> MKSRLKQQIFAISLLACTAISPANALQTHLLREQFQNPSDEAKPWTFWYWMFGAVSKEGITADLEAMKRAGLGGTYLMPIKGIKEGPQYNGKAQQLTPEWWEMVRFSMEEADRLGLKLGMHICDGFALAGGPWMTPKESMQKIVWSDTIVDGGKIKGLHLPQPEAYEGFYEDISLFALPVKEEAADVMPAQITCANIATGNHIDIKKTVNMDDAGVIRSSYPCYIQYEYEQPFTCRNIEIILSGNNYQAHRLKVMASDDGVNYRLVKQLVPARQGWQNTDENSTHAIPATTARYFRFYWTPEGSEPGSEDMDAAKWKPNLKIKELRLHREARLDQWEGKAGLVWRVASSTKKEEIGEQDCYALSQIINLTDPFKNSPSDNFKERTLTATLPKGKWKLLRMGHTATGHTNATAGGGKGLECDKFNPKAVRKQFDNWFAQAFVKTNPDVARRVLKYMHVDSWQCGSQNWSDTFAAEFRKRRGYDLMPYLPLLAGIPMESAERSEKILRDVRTTIGELVVDVFYQVLADCAKEYDCQFSAECVAPTMVSDGLLHYQKVDLPMGEFWLNSPTHDKPNDMLDAISGAHIYGKNIIQAEGFTEVRGTWNEHPGILKALLDRNYALGINRLFFHVYVHNPWLDRKPGMTLDGIGLFFQRDQTWWNKGAKAFCEYITRCQSLLQYGHPVADIAVFTGEEMPRRSILPERLVPSLPGIFGAERVESERIRLANEGQPLRVRPVGVTHSANMSDPEKWVNPLRGYAYDSFNKDALLRLAKAENGRMTLPGGASYKVLVLPLPRPMNPDPAALSPEVKQKINELKEAGILIPSLPYKEDDFSSYGLERDLIVPENIAWTHRQGEQGDIYFIANQLEETRTFTASMRIDGRKPECWNPVTGEINADIPYEQKSHRTEITLTLAPNESVFIVYPAEEDDKETSEKERKEKKDSVKEASETGLEATEYTVTFTANGKTIQRQELFDWSKEEDEQIRYYSGTAVYKTTFRWKSKVKEDQQVYLNLGKVCDLATVRVNGIDCGTIWTAPYRADITA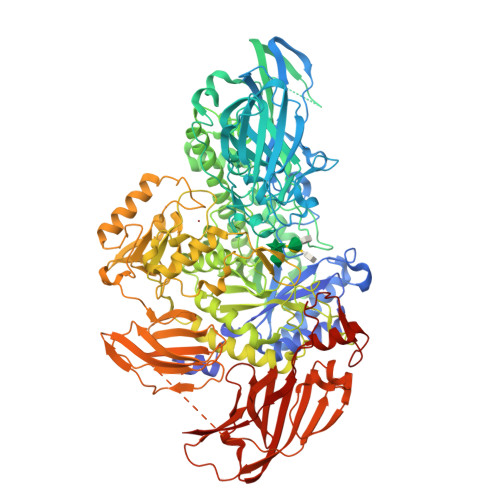ALKKGVNELEIEVTNTWANALKGADEGKAPFDGIWTNAKYRRAENTLLPAGLLGPLNFDVANKNK>MADFLLRPIKQRHRNEDKYVSVDAADGSVSKIEPIADFVIKTKLLSANGPEKLQDGRKVFINVCHSPLVPKPEVDFNARIVFPLIIQNEWEIPIITSCYRMDHDKKGQECYVWDCCINSDCSRWICDDIQLREILVEWCLESCEIRDSVVLCRDRIAFPKMKKKGAELPALEVLNDELHQDYKAK[2x]

The R2TP complex is found in organisms from yeast to humans, and consists of the AAA+ ATPases Rvb1 and Rvb2 (human: RUVBL1 and RUVBL2), a TPR-containing protein, Tah1 (human: Spagh or RPAP3), and Pih1 (also known as NOP17 and Pih1D1, but referred to as Pih1 henceforth; Kakihara and Houry, 2012; Te et al., 2007). Pih1 is the multipoint scaffold of the R2TP complex, coupling the Rvb1-Rvb2 hetero-dodecamer, the Hsp90 chaperone machinery (via Tah1 in yeast or Spagh/RPAP3 in metazoa), and the TTT (Tel2-Tti1-Tti2) complex implicated in activation and stabilization of PIKKs (Hurov et al., 2010; Kakihara and Houry, 2012). The biological roles ascribed to the R2TP complex are directly associated with its ability to interact with the Hsp90 chaperone system and function as an Hsp90 cochaperone (Boulon et al., 2010; Izumi et al., 2012; Takai et al., 2010). Here we present crystal structures of Hsp90-Tah1-Pih1, Hsp90-Spagh/RPAP3, and Pih1-Tel2 complexes that together define key structural links within the R2TP core in yeast and in animals and reveal how R2TP connects the Hsp90 chaperone system to the TTT complex involved in PIKK activation.

Interaction with Tel2 involves the N-terminal segment of Pih1 (Horejsí et al., 2010), which contains a conserved region of unknown structure (henceforth, PIH domain). We also obtained crystals of an essentially identical region of budding yeast Pih128–184 and determined the structure of this with molecular replacement. The PIH domain consists of a twisted five-stranded β sheet with one face traversed by a helix-turn-helix segment connecting strands 4 and 5, and the other face traversed by a coil segment extending from the end of β strand 5. An additional α helix connecting strands 2 and 3 projects from the end of the sheet and packs against the larger of the other two helices.> MNAPVQDAEARELALAGMGASRLRKEDARFIQGKGNYVDDIKMPGMLHMDIVRAPIAHGRIKKIHKDAALAMPGVHAVLTAEDLKPLKLHWMPTLAGDVAAVLADEKVHFQMQEVAIVIADDRYIAADAVEAVKVEYDELPVVIDPIDALKPDAPVLREDLAGKTSGAHGPREHHNHIFTWGAGDKAATDAVFANAPVTVSQHMYYPRVHPCPLETCGCVASFDPIKGDLTTYITSQAPHVVRTVVSMLSGIPESKVRIVSPDIGGGFGNKVGIYPGYVCAIVASIVLGRPVKWVEDRVENISTTAFARDYHMDGELAATPDGKILGLRVNVVADHGAFDACADPTKFPAGLFHICSGSYDIPRAHCSVKGVYTNKAPGGVAYRCSFRVTEAVYLIERMVDVLAQKLNMDKAEIRAKNFIRKEQFPYTTQFGFEYDSGDYHTALKKVLDAVDYPALRAEQAARRADPNSPTLMGIGLVTFTEVVGAGPSKMCDILGVGMFDSCEIRIHPTGSAIARMGTITQGQGHQTTYAQIIATELGIPSEVIQVEEGDTSTAPYGLGTYGSRSTPVAGAAIALAARKIHAKARKIAAHMLEVNENDLDWEVDRFKVKGDDSKFKTMADIAWQAYHQPPAGLEPGL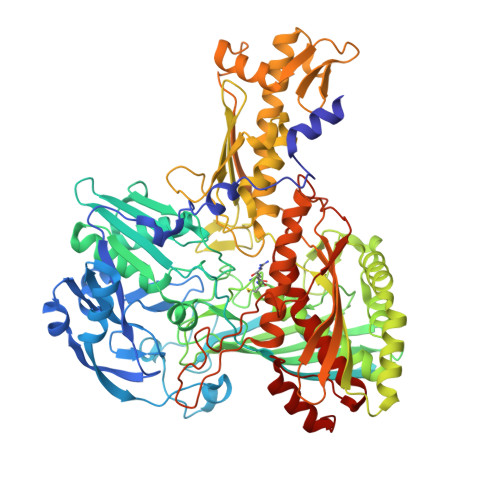EAVHYYDPPNFTYPFGIYLCVVDIDRATGETKVRRFYALDDCGTRINPMIIEGQIHGGLTEGYAVAMGQQMPFDAQGNLLGNTLMDYFLPTAVETPHWETDHTVTPSPHHPIGAKGVAESPHVGSIPTFTAAVVDAFAHVGVTHLDMPHTSYRVWKSLKEHNLAL PRSS3/Mesotrypsin is one of three tryptic digestive enzymes produced and secreted from the human pancreas. Unlike other trypsin isoforms, it possesses resistance to proteinaceous trypsin inhibitors. Additionally, mesotrypsin displays differential activity from the other two human trypsin isoforms, displaying reduced capability for activating pancreatic zymogens, reduced activation of protease activated receptors (PARs), and elevated proteolytic activity towards proteinaceous trypsin inhibitors. Mesotrypsin differs from other human trypsin family members at twenty-eight residues; Arg-193 is one of the most critical because it is located within the active site, at a position where almost all other trypsin and chymotrypsin family serine protease members possess a highly conserved glycine residue.

Upon obtaining pentamidine, we assayed the three bis-benzamidine compounds against mesotrypsin over multiple substrate and compound concentrations to determine the inhibition mode: competitive, non-competitive, or mixed inhibition. All three compounds exhibited a competitive inhibition mode of binding toward mesotrypsin (shown for diminazene in Fig 3), with inhibition constants (Ki) of 3.66, 5.10, and 10.57 μM for diminazene, pentamidine, and hydroxystilbamidine respectively. Diminazene bound to mesotrypsin most tightly while also being the least selective for the other trypsin isoforms, and was in turn selected as the best candidate compound for further investigation based on this profile. We set out to crystallize diminazene with mesotrypsin to gain a structural view of this candidate compound bound within the mesotrypsin active site. The diminazene-mesotrypsin complex crystallized in the P212121 space group having the unit cell dimensions of a = 40.92, b = 64.44, c = 80.68 and αβγ = 90°. Following refinement, well defined density was observed for the first benzamidine moiety of diminazene, which was observed to bind within the specificity pocket of mesotrypsin. In the present structure, nitrogen atoms NAA and NAC of diminazene display hydrogen bonding contacts with Asp-189 of the specificity pocket. The positioning of diminazene in the specificity pocket closely recapitulates the position predicted for the ligand by the docking screen, with a ligand RMSD of 0.614 Å. The second benzamidine moiety of the diminazene molecule exhibited diffuse density, which may be attributable to exposure to the solvent channel, permitting multiple ligand conformations. We anticipate the conformational disorder observed in diminazene could arise in part from cis-to-trans isomerization of the triazene linker. Although our high resolution crystal structure revealed the second benzamidine ring of diminazene to be poorly ordered within the mesotrypsin active site, the top ranking binding pose of this molecule from the virtual screen presented a conformational isomer with diminazene interaction at Arg-193.

> IVGGYTCEENSLPYQVSLNSGSHFCGGSLISEQWVVSAAHCYKTRIQVRLGEHNIKVLEGNEQFINAAKIIRHPKYNRDTLDNDIMLIKLSSPAVINARVSTISLPTAPPAAGTECLISGWGNTLSFGADYPDELKCLDAPVLTQAECKASYPGKITNSMFCVGFLEGGKDSCQRDSGGPVVCNGQLQGVVSWGHGCAWKNRPGVYTKVYNYVDWIKDTIAANS> MFKKLLHSLVAGLTFVAAVAAVPAHAQEADAQATVKTAVDDVLATIKGDPDLRGGNLQKVFQLVDQKIVPRADFKRTTQIAMGRFWSQATPEQQQQIQDGFKSLLIRTYAGALANVRNQTVAYKPFRAAADDTDVVVRSTVNNNGEPVALDYRVEKSPNGWKVYDINISGLWLSETYKNQFADVI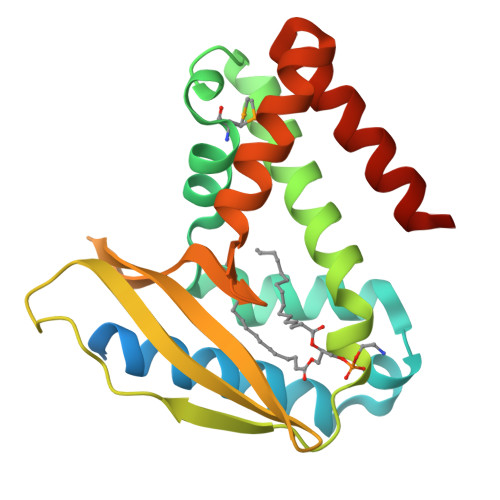SKRGGVGGLVQFLDERNAQLAKGPAK COA-S-ACETYL TRYPTAMINE | C33 H48 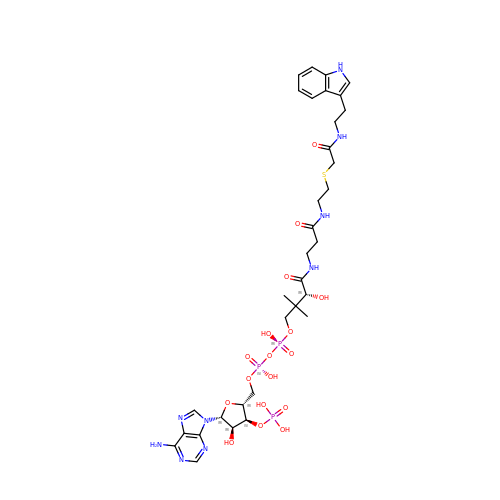N9 O17 P3 S | ZRDQFWRSRPZOSQ-GMHMEAMDSA-N>[8x]ARPTFHITVGDPHKVGDLATSHIVYSVRTKTTSKAYKQPEFEVKRRYRDFLWLYNTLHSNNPGVVVPPPPEKQAVGRFESNFVESRRAALEKMLNKIAAHPTLQLDADLKLFLESESFNIDVKHKERKEPPLGESKGVFGSLGFGGGGNKFVEQDDWFHDRRVYLDALENQLKALLKAMDNMVAQRKAMAEAAADFSASLHALSTVELSPTLSGPLDALSELQLAIRDVYERQAQQDVLTFGIIIEEYIRLIGSVKQAFSQRQKAFHSWHSAESELMKKKAAQDKLLRQGKTQQDRLNQVNAEVIDAERKVHQARLLFEDMGRLLRSELDRFEREKVEDFKSGVETFLESAVEAQKELIEKWETFLMQ;>[2x]FSTPVDIDIVLADADKRAMVDVKLDKNRREKVPLYMDGESVKGCVTVRPKDGKRLEHTGIKVQFIGTIEMFFDRGNHYEFLSLVQELAAPGELQHPQTFDF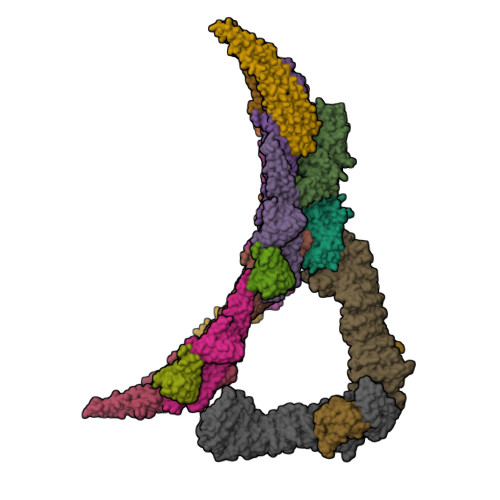NFKNVEKQYESYNGINVKLRYFVRVTVSRRMADVIREKDIWVYSYRIPPELNSSIKMDVGIEDCLHIEFEYSKSKYHLKDVIVGRIYFLLVRLKIKHMELSIIRRETTGVAPNQYNESETLVRFEIMDGSPSRGETIPIRLFLGGFDLTPTFRDVNKKFSTRYYLSLVLIDEDARRYFKQSEIILYRQPPE;>ARPTFHITVGDPHKVGDLATSHIVYSVRTKTTSKAYKQPEFEVKRRYRDFLWLYNTLHSNNPGVVVPPPPEKQAVGRFESNFVESRRAALEKMLNKIAAHPTLQLDADLKLFLESESFNIDVKHKERKE[4x];>NKFVEQDDWFHDRRVYLDALENQLKALLKAMDNMVAQRKAMAEAAADFSASLHALSTVELSPTLSGPLDALSELQLAIRDVYERQAQQDVLTFGIIIEEYIRLIGSVKQAFSQRQKAFHSWHSAESELMKKKAAQDKLLRQGKTQQDRLNQVNAEVIDAERKVHQARLLFEDMGRLLRSELDRFEREKVEDFKSGVETFLESAVEAQKELIEKWETFLMQ[2x];>RLLEDALIAVRQQTAMMRKFLDTPGKLMDALKCCSTLVSELRTSSLSPKQYYELYMAVFDALRYLSAHLRENHPVNHLADLYELVQYAGNIIPRLYLMITVGTAYMSIDGAPVKELMKDMMDMSRGVQHPVRGLFLRYYLSGQARDYLPTGDSDGPEGNLQDSINFILTNFVEMNKLWVRLQHQGHSRERDLRTQERRELQLLVGSNIVRLSQLVDLPTYRDSILGPLLEQIVQCRDILAQEYLLEVITQVFPDEYHLHTLDQFLGAVSRLNPHVNVKAIVIGMMNRLSDYAERESQNEPEEDRAKLEEEALAKLLEKTKLGQNSELEPQNGDHPDTEVSSTTDSAQAPSTADSDTTAVNGEEEPVRKRRGIPVNVPLYDIFFDQVQHLVQAQHLPIQDTIALCCSLANLSLNIYPERLDYVDGILAYALAKVKEHANSADLHSQPAQQSLLSLLQSPLRRYVSIFTALSLPTYVSLFQAQTYPTRRAIAGEIVRTLLKNQTLISTPAHLENVLEILKVLIKEGSQPPAGYPGVVQPRARPLETDETMEEQGWLARLVHLIHSDDNDTQFRLLQMTRKAYAEGNERIRTTTPPLITAGLKLARRFKAREHYDDNWSSQSSSLFKFLHSAISTLYTRVNGPGVADLCLRLFCSCGQVADMTEFEEVAYEFFAQAFTVYEESISDSKAQFQAVCVIASALHRTRNFGRENYDTLITKCAQHASKLLRKPDQCRAVYLASHLWWATPIAARGETEDTELYRDGKRVLECLQRALRVADSCMETATSIELFVEILDRYVYYFDQRNESVTTKYLNGLIELIHSNLAGNQQDSASVEASRKHFIQTLEMIQ[2x];>AFLILVIGNLHIPDRALDIPPKFKKLLSPGKISQTLCLGNLTDRATYDYLRSISPDLKIVRGRMDVEATSLPLMQVVTHGSLRIGFLEGFTLVSEEPDVLLAEANKLDVDVLCWAGGSHRFECFEYMDKFFVNPGSATGAFTTDWLAEGEEVVPSFCLMDVQGISLTLYVYQLRKDENGTENVAVEKVTYTKP[2x]Determining their respective contributions has been complicated by the previously reported association of OmcS, a cytochrome known to participate in some forms of extracellular electron exchange, with conductive filaments. We conclude that these thick filaments are not simply associated with OmcS, but rather consist of OmcS monomers, thereby representing the first example, to our knowledge, of nanowires composed entirely of a bacterial cytochrome. The unexpected filamentous assembly of a c-type cytochrome in our structure suggests new possibilities for long-range biological electron transfer.

Individual filament segments were extracted from cryo-EM images of conductive e-pili preps and, after analysis, the resulting 3D reconstruction produced a map at 3.4 Å resolution with extensive contiguous polypeptide density that could not satisfactorily fit with any combination of PilA monomers and also showed multiple regions of density along the filament providing excellent fits to c-type heme molecules. In subsequent fitting attempts using the sequences of several related Geobacter cytochromes, only that of OmcS provided a near ideal fit to the density, incorporating the full OmcS sequence corresponding to the 47.5 Å filament repeat and accounting for all 6 hemes per OmcS monomer. Each monomer repeat extends ~4.8 nm along the fiber axis, is rotated 83° and is ~4 nm wide except at the intermonomer interfaces, where the fiber narrows substantially. At the core of the fiber is a continuous, unbranched stack of hemes. Successive hemes, approaching edge-to-edge, alternate between lying parallel and perpendicular to the previous heme. The interatomic contact distances are all ≤4.1 Å. The OmcS sequence includes six Cys-x-x-Cys-His motifs, with both Cys sulfur atoms covalently attached to heme substituents, and His as one of the axial ligands. All 12 heme-axial ligands are histidine side chains, with 11 coming from the same OmcS subunit, and 1 (attached to heme505) from a neighboring molecule. Notable exceptions, which are solvent-exposed edge-on, include heme502 (from one OmcS subunit) and heme506 (from the adjacent subunit), which are both located near the narrow, intersubunit interfaces (on opposite sides of the fiber). Each OmcS monomer also includes one octahedrally coordinated metal, tentatively identified as Mg++ based on its density level and experiment, whose biological significance is unclear.

> FHSGGVAECEGCHTMHNSLGGAVMNSATAQFTTGPMLLQGATQSSSCLNCHQHAGDTGPSSYHISTAEADMPAGTAPLQMTPGGDFGWVKKTYTWNVRGLNTSEGERKGHNIVAGDYNYVADTTLTTAPGGTYPANQLHCSSCHDPHGKYRRFVDGSIATTGLPIKNSGSYQNSNDPTAWGAVGAYRILGGTGYQPKSLSGSYAFANQVPAAVAPSTYNRTEATTQTRVAYGQGMSEWCANCHTDIHNSAYPTNLRHPAGNGAKFGATIAGLYNSYKKSGDLTGTQASAYLSLAPFEEGTADYTVLKGHAKIDDTALTGADATSNVNCLSCHRAHASGFDSMTRFNLAYEFTTIADASGNSIYGTDPNTSSLQGRSVNEMTAAYYGRTADKFAPYQRALCNKCHAKD> SMLPRLICINDYEQHAKSVLPKSIYDYYRSGANDEETLADNIAAF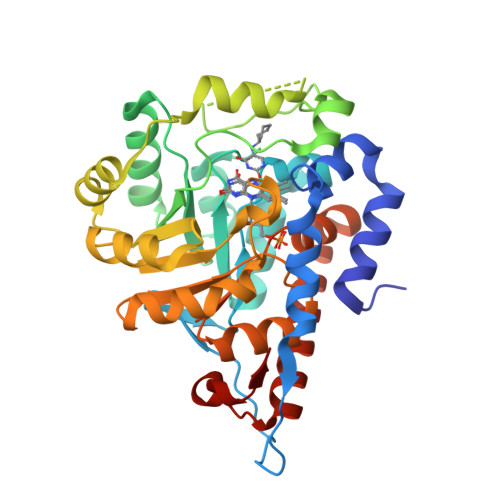SRWKLYPRMLRNVAETDLSTSVLGQRVSMPICVGATAMQRMAHVDGELATVRACQSLGTGMMLSSWATSSIEEVAEAGPEALRWLQLYIYKDREVTKKLVRQAEKMGYKAIFVTVDTPYLGNRLDDVRNRFKLPPQLRMKNFETSTLSFSPEENFGDDSGLAAYVAKAIDPSISWEDIKWLRRLTSLPIVAKGILRGDDAREAVKHGLNGILVSNHGARQLDGVPATIDVLPEIVEAVEGKVEVFLDGGVRKGTDVLKALALGAKAVFVGRPIVWGLAFQGEKGVQDVLEILKEEFRLAMALSGCQNVKVIDKTLVRKNPLAVS>[2x]MVLYFIGLGLYDERDITVKGLEIAKKCDYVFAEFYTSLMAGTTLGRIQKLIGKEIRVLSREDVELNFENIVLPLAKENDVAFLTPGDPLVATTHAELRIRMKRAGVESYVIHAPSIYSAVGITGLHIYKFGKSATVAYPEGNWFPTSYYDVIKENAERGLHTLLFLDIKAEKRMYMTANEAMELLLKVEDMKKGGVFTDDTLVVVLARAGSLNPTIRAGYVKDLIREDFGDPPHILIVPGKLHIVE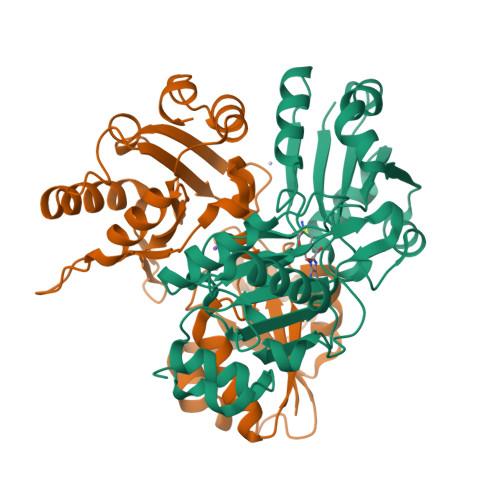AEYLVEIAGAPREILRVNV> PILKRTIISKRKAPSNNEDEEIVKTPRKLVNYVPLKIFNLGDSFDDTITTTVAKLQDLKKEILDSPRSNKSIVITSNTVAKSELQKS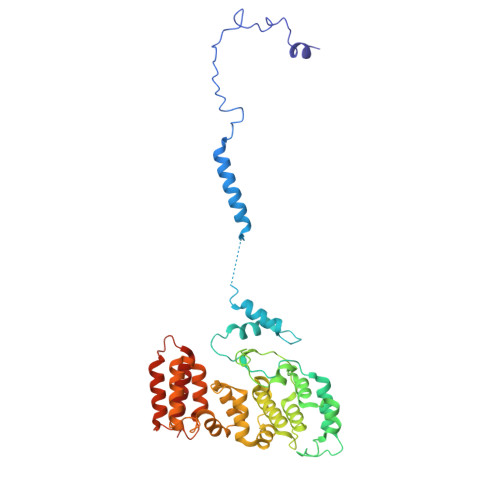IKFSGSIPEIYLDVVTKETISDKYKDWHFISKNCHYEQLMDLEMKDTAYSFLFGSSRSQGKVPEFVHLKCPSITNLLVLFGVNQEKCNSLKINYEKKENSRYDNLCTIFPVNKMLKFLMYFYSDDDNDDVREFFLKAFICLILDRKVFNAMESDHRLCFKVLELFNEAHFINSYFEIVDKNDFFLHYRLLQIFPHLQSALLRRRFSEKQGRTETIQQNIIKEFNEFFDCKNYKNLLYFILTMYGSKFIPFGPKCQVTEYFKDCILDISNETTNDVEISILKGILNLFSKIR>[2x]MPVLENRAAQGDITAPGGARRLTGDQTAALRDSLSDKPAKNIILLIGDGMGDSEITAARNYAEGAGGFFKGIDALPLTGQYTHYALNKKTGKPDYVTDGAASATAWSTGVKTYNGALGVD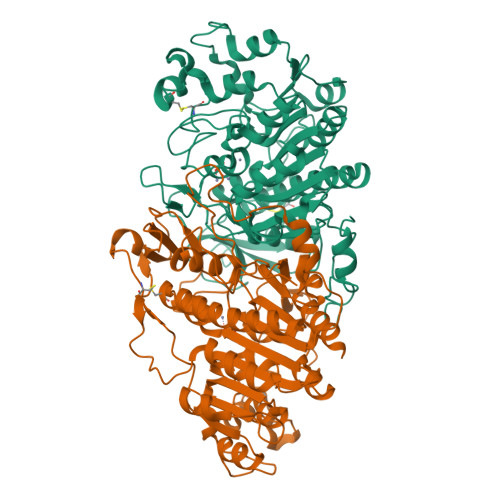IHEKDHPTILEMAKAAGLATGNVSTAELQDATPAALVAHVTSSKCYGPSATSEKCPGNALEKGGKGSITEQLLNARADVTLGGGAKTFAETATAGEWQGKTLREQAQARGYQLVSDAASLNSVTEANQQKPLLGLFADGNMPVRWLGPKATYHGNIDKPAVTCTPNPQRNDSVPTLAQMTDKAIELLSKNEKGFFLQVEGASIDKQDHAANPCGQIGETVDLDEAVQRALEFAKKEGNTLVIVTADHAHASQIVAPDTKAPGLTQALNTKDGAVMVMSYGNSEEDSQEHTGSQLRIAAYGPHAANVVGLTDQTDLFYTMKAALGL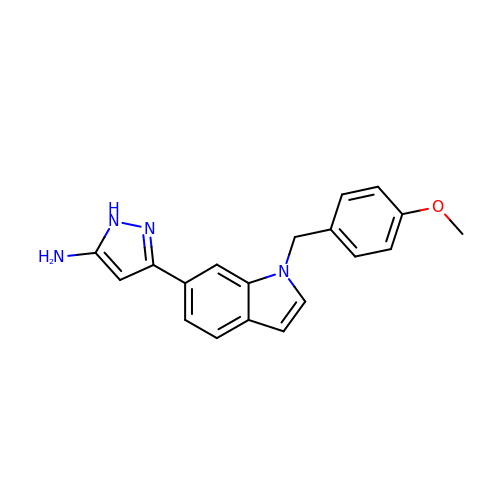3-[1-[(4-methoxyphenyl)methyl]indol-6-yl]-1~{H}-pyrazol-5-amine | C19 H18 N4 O | OQIZQMWQHPDPIM-UHFFFAOYSA-N> KQ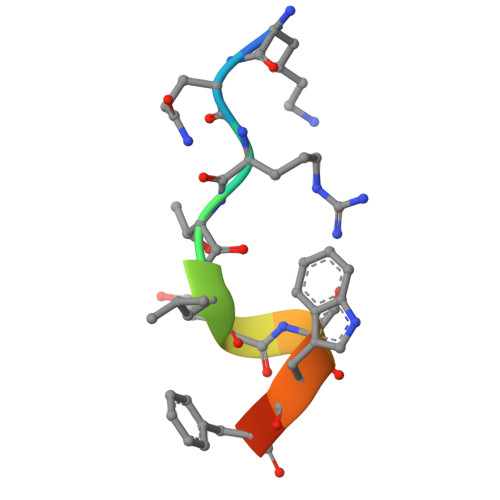RTLESWFGR>[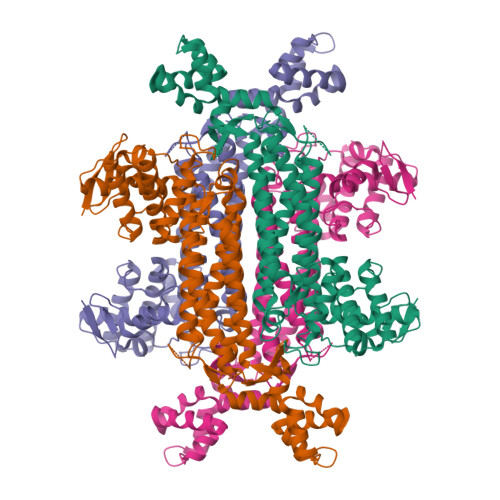4x]GAVDADSANYRIEHDTMGEVRVPAKALWRAQTQRAVENFPISGRGLERTQIRALGLLKGACAQVNSDLGLLAPEKADAIIAAAAEIADGQHDDQFPIDVFQTGSGTSSNMNTNEVIASIAAKGGVTLHPNDDVNMSQSSNDTFPTATHIAATEAAVAHLIPALQQLHDALAAKALDWHTVVKSGRTHLMDAVPVTLGQEFSGYARQIEAGIERVRACLPRLGELAIGGTAVGTGLNAPDDFGVRVVAVLVAQTGLSELRTAANSFEAQAARDGLVEASGALRTIAVSLTKIANDIRWMGSGPLTGLAEIQLPDLQPGASIMPGKVNPVLPEAVTQVAAQVIGNDAAIAWGGANGAFELNVYIPMMARNILESFKLLTNVSRLFAQRCIAGLTANVEHLRRLAESSPSIVTPLNSAIGYEEAAAVAKQALKERKTIRQTVIDRGLIGDRLSIEDLDRRLDVLAMAKAEQLDSDRL>[2x]MTDSA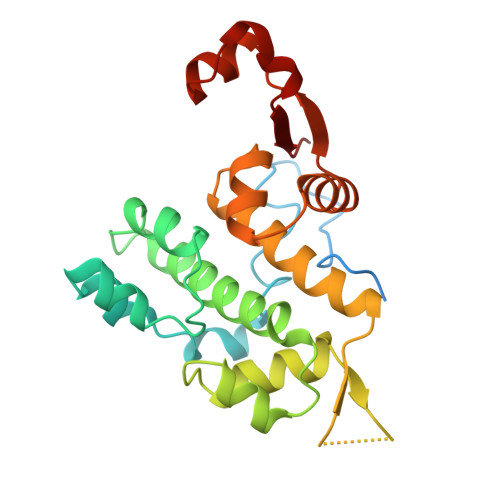IDIVDSVRTASKDLPTRAQLDEITSNDRPTPLANIDATDVEQIYPIESIIPKKELQFIRVSSILKEADKEKKLELFPYQNNSKYVAKKLDSLTQPSQMTKLQLLYYLSLLLGVYENRRVNNKTKLLERLNSPPEILVDGILSRFTVIKPGQFGRSKDRSYFIDPQNEDKILCYILAIIMHLDNFIVEITPLAHELNLKPSKVVSLFRVLGAIVKGATVAQAEAFGIPKSTAASYKIATMKV The AmpC type class C SBLs, unlike many β-lactamases, are chromosomally encoded and present in most E. coli strains. Mutations in promoter and attenuator regions lead to hyperproduction of AmpC in pathogenic E. coli, conferring resistance to first-, second-, and third-generation cephalosporins and most penicillins, although as yet not to carbapenems. We report kinetic and structural studies, including four high-resolution crystal structures, concerning inhibition of the AmpC serine-β-lactamase from E. coli (AmpCEC) by clinically relevant DBO-based inhibitors: avibactam, relebactam, nacubactam, and zidebactam. Contrary to the proposed mechanisms of the established β-lactam SBL inhibitors, which involve essentially irreversible formation and subsequent hydrolysis of acyl-enzyme complexes, the cyclic urea carbonyl of avibactam reacts reversibly with the nucleophilic serine residue to form a carbamoyl-enzyme complex.

In reported structures of AmpC-DBO complexes, the orientation of the N-sulfate nitrogen can adopt two conformations. In one (conformation A), the N-sulfate nitrogen is close to the Y150 phenol sidechain, while in the other (conformation B) the nitrogen atom points toward the opposite face of the active site. For REL and ZID, both conformations A and B were observed and refined in equal occupancy. The N-sulfate nitrogen is 3.8 and 3.5 Å from Y150:Oη in conformation A and 4.7 and 4.8 Å from Y150:Oη in conformation B for REL and ZID, respectively. While the αBD angles are comparable in both conformations A and B (112° to 115°), the orientation of the N-sulfate nitrogen is stereoelectronically unfavorable for reaction with the carbamoyl carbonyl group in conformation B, where the distance to the carbamoyl carbon is significantly increased compared to that of conformation A (3.9 Å compared to 3.0 Å for REL and 3.8 Å compared to 2.8 Å for ZID). However, in the case of the REL- and ZID-derived complexes, only approximately half of the molecules are in the productive conformation (A), while the other half adopt conformation B, in which the N-sulfate nitrogen lone pair is directed away from the reactive carbonyl group. Based on the proposed decarbamoylation mechanisms of DBOs for class C SBLs and stereoelectronic considerations of the mechanism of the nucleophilic attack, the REL- and ZID-derived complexes appear less primed for recyclization, since they form both conformations A and B, than those of AVI and NAC, where only conformation A is observed. The piperidyl nitrogen does not appear to engage in any direct or water-mediated hydrogen bonding interactions with AmpCEC active-site residues. The Ω-loop and H-10 helix are located at the R2 binding pocket of the active site, and the different acyl-amido sidechains of REL, NAC, and ZID, which are positioned in this pocket, are likely to have an impact on inhibition of those AVI-resistant mutants.

> APQQINDIVHRTITPLIEQQKIPGMAVAVIYQGKPYYFTWGYADIAKKQPVTQQTLFELGSVSKTFTGVLGGDAIARGEIKLSDPTTKYWPELTAKQWNGITLLHLATYTAGGLPLQVPDEVKSSSDLLRFYQNWQPAWAPGTQRLYANSSIGLFGALAVKPSGLSFEQAMQTRVFQPLKLNHTWINVPPAEEKNYAWGYREGKAVHVSPGALDAEAYGVKSTIEDMARWVQSNLKPLDINEKTLQQGIQLAQSRYWQTGDMYQGLGWEMLDWPVNPDSIINGSDNKIALAARPVKAITPPTPAVRASWVHKTGATGGFGSYVAFIPEKELGIVMLANKNYPNPARVDAAWQILNALQ>[2x]MLTMKDI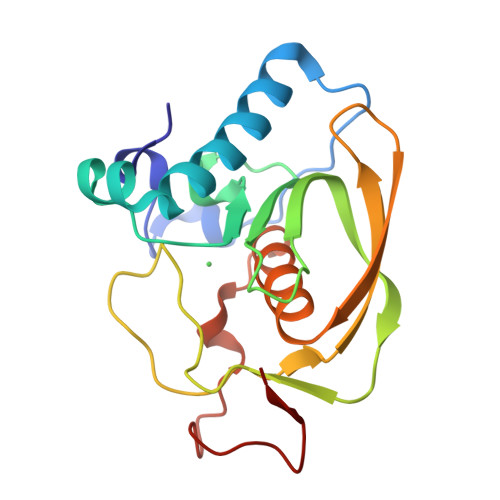IRDGHPTLRQKAAELELPLTKEEKETLIAMREFLVNSQDEEIAKRYGLRSGVGLAAPQINISKRMIAVLIPDDGSGKSYDYMLVNPKIVSHSVQEAYLPTGEGCLSVDDNVAGLVHRHNRITIKAKDIEGNDIQLRLKGYPAIVFQHEIDHLNGVMFYDHIDKNHPLQPHTDAVEV>MAHHHHHHMSRLIVVSNRVAAGEDTRPSAGGLAVGVMDALKQTGGVWFGWNGEIVGTPDAAPAVRRDGNVTYATLGLTRRDYDQYYRGFSNATLWPVFHYRSDLARFDRQEYAGYLRVNAMLARQLAALLRPDDLIWVHDYHLLPFAHCLRELGVKNPIGFFLHIPFPSPDMLRVVPPHDELVKFMCAYDIAGFQTDADKRAFSDYIERRGIGTASDDGMLHAHGRVVKVAAYPIGVYPDAIAEAAVQYGGRKPVKMLRDALGGRKLVMSVDRLDYSKGLVERFQSFERMLAGAPDW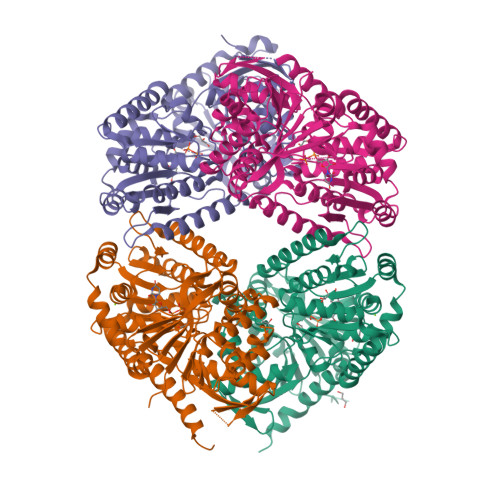QGRVSFVQIAPPTRSDVQTYQRIRETLEREAGRINGRFAQLDWTPIQYLNRKYERNLLMAFFRMSQVGYVTPLRDGMNLVAKEYVASQDPADPGVLVLSEFAGAAAELGGALLVNPYDHAQMADALARALAMPLAERQARHEENLAQLRNNDLSVWRDTFVADLRSVAAAASVTQRAGRRTAHV[8x]(2R,3S,4S,5S,6R)-2-((2S,3S,4R,5R,6R)-5-AMINO-2-(AMINOMETHYL)-6-((2R,3S,4R,5S)-5-((1R,2R,3S,5R,6S)-3,5-DIAMINO-2-((2S,3R,5S,6R)-3-AMINO-5-HYDROXY-6-(HYDROXYMETHYL)-TETRAHYDRO-2H-PYRAN-2-YLOXY)-6-HYDROXYCYCLOHEXYLOXY)-4-HYDROXY-2-(HYDROXYMETHYL)-TETRAHYDROFURAN-3-YLOXY)-4-HYDROXY-TETRAHYDRO-2H-PYRAN-3-YLOXY)-6-(HYDROXYMETHYL)-TETRAHYDRO-2H-PYRAN-3,4,5-TRIOL 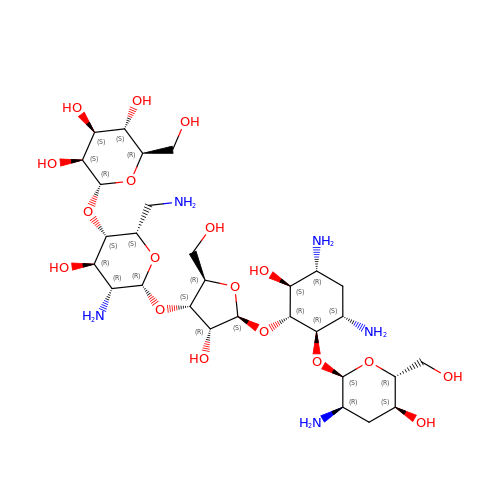| C29 H55 N5 O18 | DBLVDAUGBTYDFR-SWMBIRFSSA-N>SNAMDGMTIDWSGVAAAVAAAEATGGTVGATIVAPGGETFRHNGDRRFRAASTVKIPLMIAVYRAVDAGERALTDRIVLRAADKAPGSGVLLHLHDG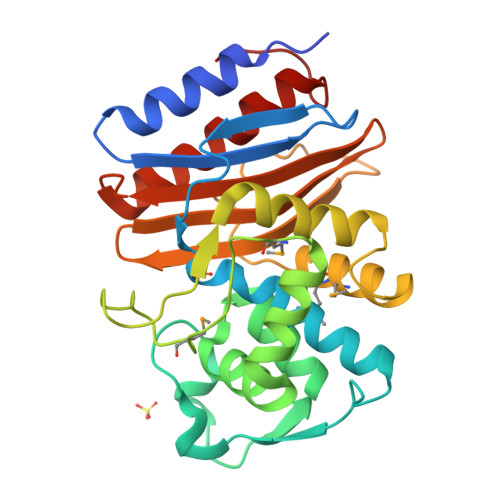LELTLEDLVYLTISISDNTATNLLIDLVGLDAVNDVIASLGMRDSNLSRKMKGRPALPDEPENWATPDDYALAVQALLEGRAASQESCTAMLAMLEKQQNPRRIGRYVPEGEGIRWGSKTGSLTGVVNDVGFITTPAGTLVVAVFTENLPDLHAGEQAIGDITRAALQATGLIPPGAA[4x]> GPLGSMPGFSQATELGAWKELQEHHNSLGRNIVLKEYFEKDPQRFEKFSRTFANPVDNTEILFDFSKNFLTEETLALLVKLAREAGVEELRDAMFKGDPINFTEDRAVYHVALRNVTNEPMQVNGKSVVEDVNSVLEHMKEFTEQVRSGEWKGYTGKKITTIINIGIGGSDLGPVMVTEALKPYGAEDMTLHFVSNIDGSHIAEALKHSDPETTLFLIASKTFTTAETTTNANSAKKWFLESAKDEAHIAKHFVALSTNEEEVTKFGIDKKNMFGFASWVGGRYSVWSAIGLSVALYIGFDNFHQFLAGAHAMDKHFRETPLEQNIPVLGGLLSVWYSDFFGAQTHLVAPFDQYLHRFPAYLQQLSMESNGKAITRTGEYVKYTTGPILFGEPATNAQHSFFQLLHQGTKLIPSDFIMAAESHNPVEGGKHQRMLASNFLAQSEALMVGKTPEQVKTEGAPDNLVPHKTFLGNRPTTSILAQKITPSTLGALIAYYEHLTFTEGAVWNINSFDQWGVELGKVLAKKIQKELETPGAGGDHDASTSGLLLAFKKKANLA

Phosphoglucose isomerase (PGI; EC 5.3.1.9) catalyzes the reversible conversion of fructose-6-phosphate (Fru6P) to glucose-6-phosphate (Glc6P). Furthermore, Glc6P can be converted to UDP-Glc, whereas Fru6P can be converted to UDP-GlcNAc and GDP-Man. These three nucleotide sugars are the main precursor molecules for all cell wall carbohydrates, including chitin (UDP-GlcNAc), galactomannan (GDP-Man), and glucan (UDP-Glc). The AfPGI protein contains 553 amino acids with 71, 57, and 56% identity to Candida albicans PGI (CaPGI, P83780), C. neoformans PGI (CnPGI, Q5KLU5), and Homo sapiens PGI (HsPGI, P06744), respectively.

AfPGI was also crystallized in the same condition without Glc6P, and the apo structure of AfPGI was solved by molecular replacement using the AfPGI-Glc6P complex structure as the search model and refined to 1.56 Å with an Rwork/Rfree value of 15.7/18.3. However, we unexpectedly observed that a citrate molecule (buffer component) binds to the gateway of the active site and is also recognized by the phosphate-binding loop in the apo AfPGI structure. The phosphate-binding loop adopts an “open” conformation compared to the structure of AfPGI-Glc6P complex and therefore places the citrate molecule proximal (5 Å) to Ala221, suggesting that the gateway between the active site and Ala221 is ligandable. Compounds bound to the gateway are potential starting points to explore specific fungal inhibitors. The intrinsic flexibility of lysine implies that the Lys520 sidechain is likely to move away from the gap, in agreement with the fact that there is no electron density around the Lys520 sidechain in the structure of apo AfPGI. This intrinsic mobility of Lys520 could leave an empty gap between Ala221 and Gln523.>[12x]MEFKKVAKETAITLQSYLTYQAVRLI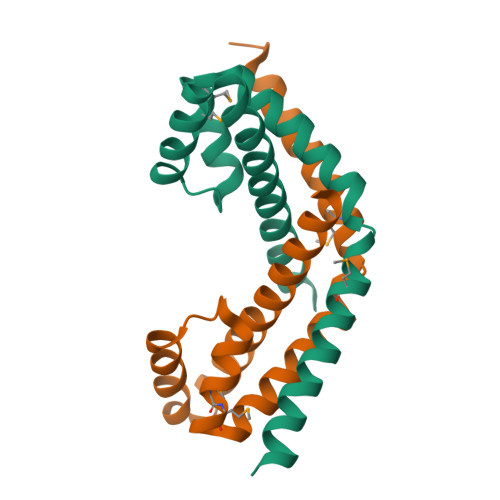SQQLSETNPGQAIWLGEFSKRHPIQESDLYLEAMMLENKELVLRILTVRENLAEGVLEFLPEMVLSQIKQSNGNHRRSLLERL>GSHMGEKRSIAIDSYQEDPSVVVSNFFKGVRVPKDTEFQLYKKRKQDQFVLHGENERLEYDGETDELTTKTNQYMVGLYDKQSGKINLYRAPVVTSKIVSKFSKNLKGPEIKSKGDTRYGAM[4x];>MGYQPPSDYKQCKHLKSFPVSELKGDNKELWLMKVPANIDISQLKSLPLDTDATVSTVELGSKNFNVLQNTSTQEGSDNTNLSLLIPSEKKKETLKVATSKDNKSVYFDRVFTISETARIP[4x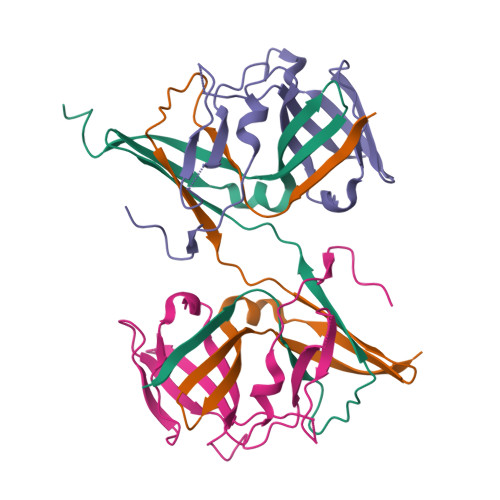]>[6x]MDSNDLEASFTSRLPPEIVAALKRKSSRDPNSRFPRKLHMLLTYLASNPQLEEEIGLSWISDTEFKMKKKNVALVMGIKLNTLNVNLRDLAF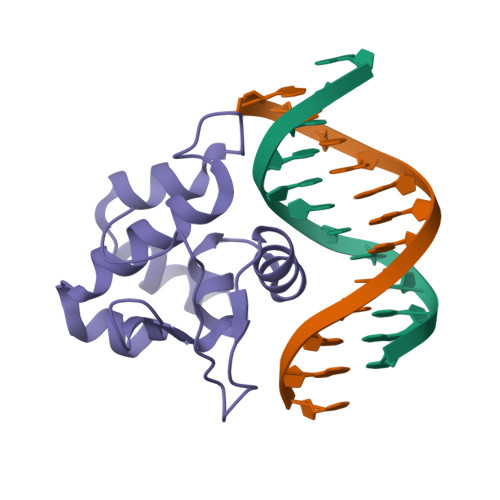EQLQHDKGGWTQWKRSGFTRNSVFEDPTQNDSPMHHHHHH>MASGTTTTAVKIGIIGGTGLDDPEILEGRTEKYVDTPFGKPSDALILGKIKNVDCVLLARHGRQHTIMPSKVNYQANIWALKEEGCTHVIVTTACGSLREEIQPGDIVIIDQFIDRTTMRPQSFYDGSHSCARGVCHIPMAEPFCPKTREVLIETAKKLGLRCHSKGTMVTIEGPRFSSRAESFMFRTWGADVINMTTVPEVVLAKEAGICYASIAMATDYDCWKEHEEAVSVDRVLKTLKENANKAKSLLLTTIPQIGSTEWSE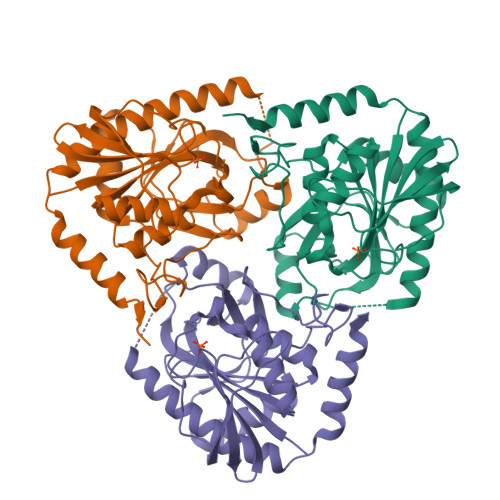TLHNLKNMAQFSVLLPRH[6x]> MEQRSAETRIVEALLERRRLKDTDLLRARQLQAESGMGLLALLGRLGLVSERDHAETCAEVLGLPLVD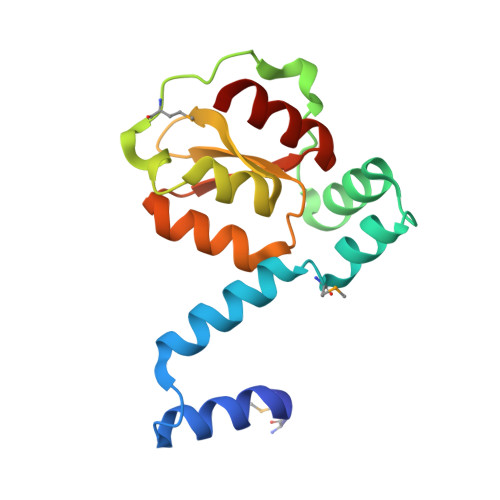ARQLGDTPPEMLPEVQGLSLRFLKQFHLCPVGERDGRLDLWIADPYDDYAIDAVRLATGLPLLLHVGLRSEIDDLIERWYG>MTIFQFPQDFMWGTATAAYQIEGAYQEDGRGLSIWDTFAHTPGKVFNGDNGNVACDSYHRYEEDIRLMKELGIRTYRFSVSWPRIFPNGDGEVNQKGLDYYHRVVDLLNDNGIEPFCTLYHWDLPQALQDAGGWGNRRTIQAFVQFAETMFREFHGKIQHWLTFNEPWCIAFLSNMLGVHAPGLTNLQTAIDVGHHLLVAHGLSVRRFRELGTSGQIGIAPNVSWAVPYSTSEEDKAACARTISLHSDWFLQPIYQGSYPQFLVDWFAEQGATVPIQDGDMDIIGEPIDMIGINYYSMSVNRFNPEAGFLQSEEINMGLPVTDIGWPVESRGLYEVLHYLQKYGNIDIYITENGACINDEVVN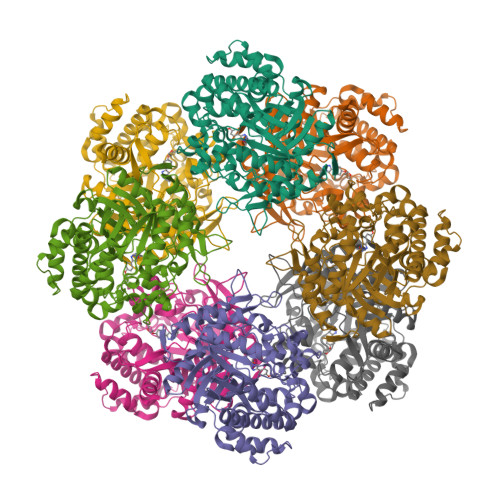GKVQDDRRISYMQQHLVQVHRAIHDGLHVKGYMAWSLLDNFEWAEGYSMRFGIIHVDFRTQVRTPKESYYWYRKVVGNNWLETRR[2x]9ALPHA-FLUOROCORTISOL | C21 H29 F O5 | 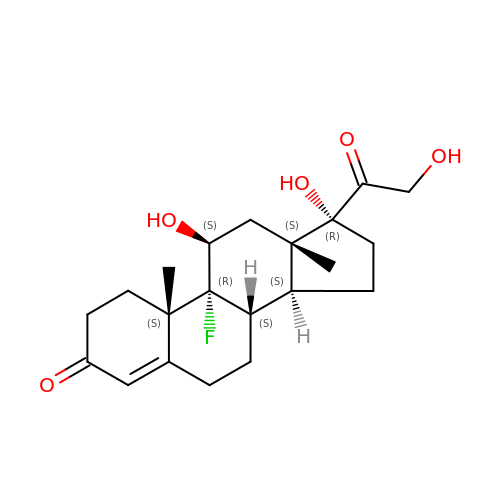AAXVEMMRQDVLJB-BULBTXNYSA-N>[3x]HHHHHHSGNTIVNGAPAINASLNIAKSETKVYTGEGVDSVYRVPIYYKLKVTNDGSKLTFTYTVTYVNPKTNDLGNISSM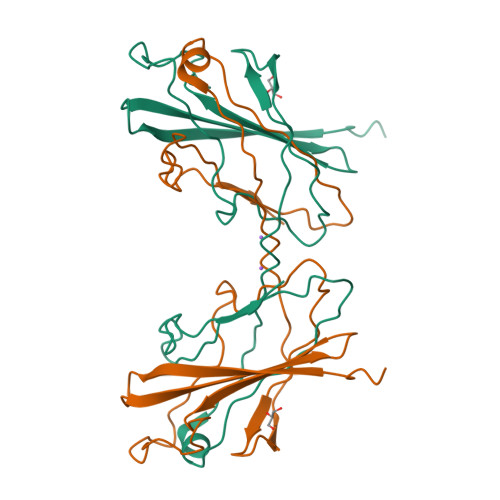RPGYSIYNSGTSTQTMLTLGSDLGKPSGVKNYITDKNGRQVLSYNTSTMTTQGSGYTWGNGAQMNGFFAKKGYGLTSSWTVPITGTDTSFTFTPYAARTDRIGINYFNGGGKVVESST> MNNTFKFLHQVISKLTLKAQVPNYGQYSHSLKRPINPKVVVFGNSSRAYELISSQFRNFNHVNGLELKGQEDNIQANKVAQSVLSINDGFQDGYYITDFPQNS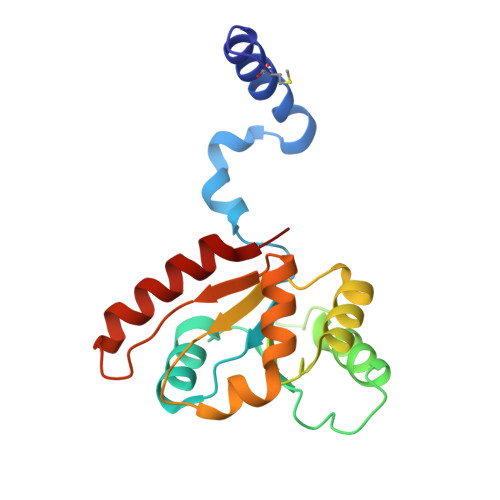KQAERLDLITDGVNLALYIKDPSDKVTVTRQQEAIDYYRKTGALVEFEVDPRGDLEEQVKQLSNQVLNGYKH2-[(2R)-butan-2-yl]-4-{4-[4-(4-{[(2R,4S)-2-(2,4-dichlorophenyl)-2-(1H-1,2,4-triazol-1-ylmethyl)-1,3-dioxolan-4-yl]methoxy}phenyl)piperazin-1-yl]phenyl}-2,4-dihydro-3H-1,2,4-triazol-3-one | C35 H38 Cl2 N8 O4 | 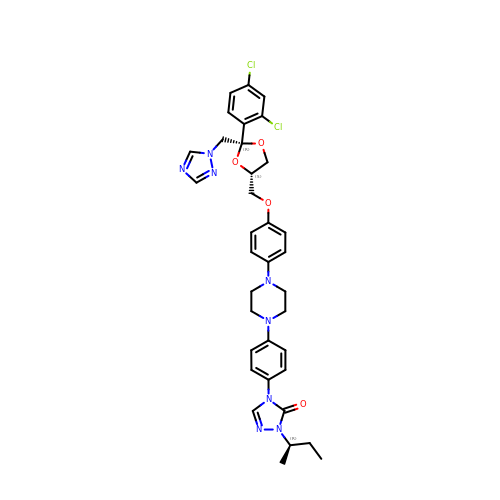VHVPQPYKVGDNFY-DFMJLFEVSA-N>[6x]DVTVVYQNGLP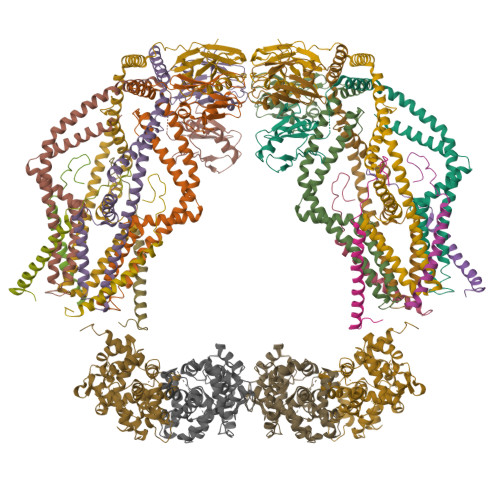VISVRLPSRRERCQFTLKPISDSVGVFLRQLQEEDRGIDRVAIYSPDGVRVAASTGIDLLLLDDFKLVINDLTYHVRPPKRDLLSHENAATLNDVKTLVQQLYTTLCIEQHQLNKERELIERLEDLKEQLAPLEKVRIEISRKAEKRTTLVLWGGLAYMATQFGILARLTWWEYSWDIMEPVTYFITYGSAMAMYAYFVMTRQEYVYPEARDRQYLLFFHKGAKKSRFDLEKYNQLKDAIAQAEMDLKRLRDPLQVHLPLRQ;>[8x]VIVTRSGAILPKPVKMSFGLLRVFSIVIPFLYVGTLISKNFAALLEEHDIFVP;>[2x]DVTVVYQNGLPVISVRLPSRRERCQFTLKPISDSVGVFLRQLQEEDRGIDRVAIYSPDGVRVAASTGIDLLLLDDFKLVINDLTYHVRPPKRDLLSHENAATLNDVKTLVQQLYTTLCIEQHQLNKERELIERLEDLKEQLAPLEKVRIEISRKAEKRTTLVLWGGLAYMATQFGILARLTWWEYSWDIMEPVTYFITYGSAMAMYAYFVMTRQEYVYPEARDRQYLLFFHKGAKKSRFDLEKYNQLKDAIAQAEMDLKRLRDPLQVH;>[2x]SGFRDRKVMEYENRIRAYSTPDKIFRYFATLKVISEPGEAEVFMTPEDFVRSITPNEKQPEHLGLDQYIIKRFDGKKISQEREKFADEGSIFYTLGECGLISFSDYIFLTTVLSTPQRNFEIAFKMFDLNGDGEVDMEEFEQVQSIIRSQTSMGMRHRDRPTTGNTLKSGLCSALTTYFFGADLKGKLTIKNFLEFQRKLQHDVLKLEFERHDPVDGRITERQFGGMLLAYSGVQSKKLTAMQRQLKKHFKEGKGLTFQEVENFFTFLKNINDVDTALSFYHMAGASLDKVTMQQVARTVAKVELSDHVCDVVFALFDCDGNGELSNKEFVSIMKQRLM;>[2x]LRKQRFMQFSSLEHEGEYYMTPRDFLFSVMFEQMERKTSVKKLTKKDIEDTLSGIQTAGCGSTFFRDLGDKGLISYTEYLFLLTILTKPHSGFHVAFKMLDTDGNEMIEKREFFKLQKIISKQDDLMTVKTNETGYQEAIVKEPEINTTLQMRFFGKRGQRKLHYKEFRRFMENLQTEIQEMEFLQFSKGLSFMRKEDFAEWLLFFTNTENKDIYWKNVREKLSAGESISLDEFKSFCHFTTHLEDFAIAMQMFSLAHRPVRLAEFKRAVKVATGQELSNNILDTVFKIFDLDGDECLSHEEFLGVLKNR> MVADSRLPNFRALTPAQRRDFLADACGLSDAERALLAAPGALPLALADGMIENVFGSFELPLGVAGNFRVNGRDVLVPMAVEEPSVVAAASYMAKLAREDGGFQTSSTLPLMRAQVQVLGVTDPHGARLAVLQARAQIIERANSRDKVLIGLGGGCKDIEVHVFPDTPRGPMLVVHLIVDVRDAMGANTVNTMAESVAPLVEKIT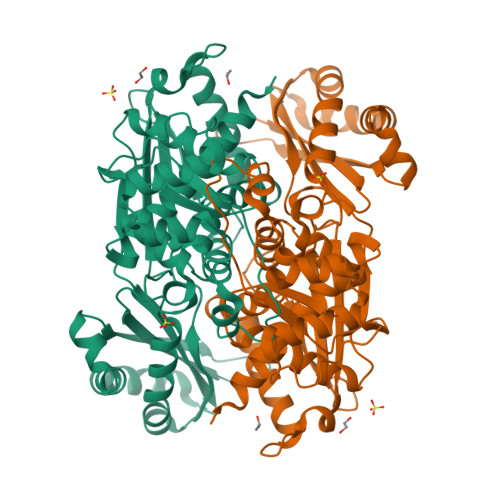GGSVRLRILSNLADLRLARARVRLTPQTLATQDRSGEEIIEGVLDAYTFAAIDPYRAATHNKGIMNGIDPVIVATGNDWRAVEAGAHAYASRSGSYTSLTRWEKDAGGALVGSIELPMPVGLVGGATKTHPLARLALKIMDLQSAQQLGEIAAAVGLAQNLGALRALATEGIQRGHMALHARNIALVAGATGDEVDAVARQLAAEHDVRTDRALEVLAALRARA> NGVELSAVGVLLPVLMDSGRRISGGAFMAVKGDLSEHIKNPKNTRIAQTVAGGTIYGLSEMVNIDEAEKLPIKGAITVLPVVQATATSILVPDNQPQLAFNSWEAAACAADTLESQQTPFLMVTGAVESGNLSPNLLAV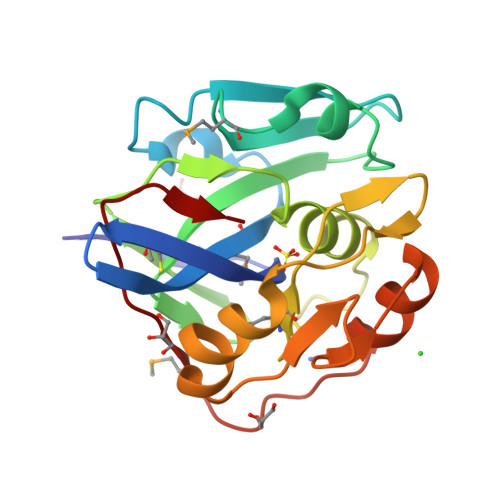QKQLLVAKPAGIGLAANSDRALKVVTLEQLRQVVGDKPWRKPMVTFSSGKNVAQA>MSNTKTASTGFAELLKDRREQVKMDHAALASLLGETPETVAAWENGEGGELTLTQLGRIAHVLGTSIGALTPPAGNDLDDGVIIQMPDERPILKGVRDNVDYYVYNCLVRTK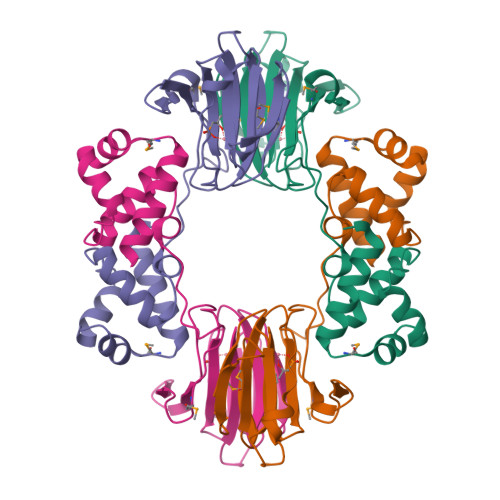RAPSLVPLVVDVLTDNPDDAKFNSGHAGNEFLFVLEGEIHMKWGDKENPKEALLPTGASMFVEEHVPHAFTAAKGTGSAKLIAVNF[2x]>[2x]GMTDTNLVEMRAIERMMFDYSYHLDMNHPEELAALFVEDCEVSYAPNFGATGRDAYKKTLEGIGTFFRGTSHHNSNICIDFVSETEANVRSVVL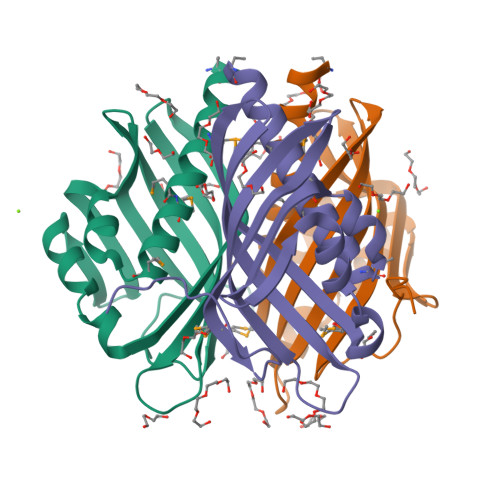AIHRYTKERPDGILYGQYFDTVVKVDGQWKFKRRELRTTMTTDYHVRAANPIGRAE> SAW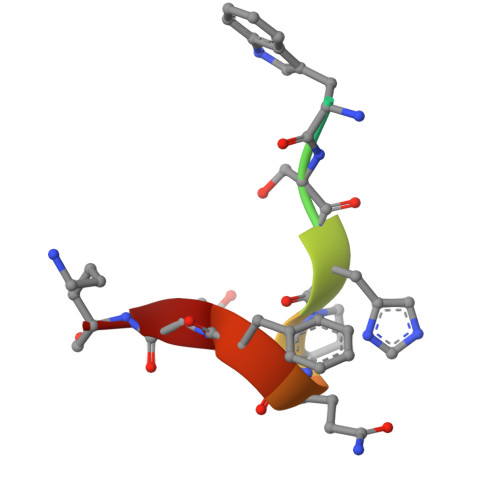SHPQFEK>AYLLFYTEAKVALAVK[12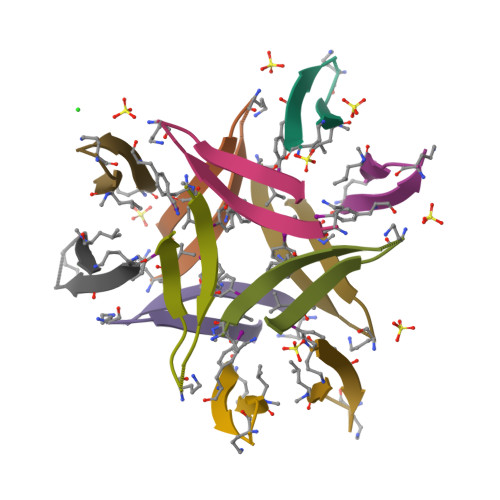x]>ASCPGACVCYNEPKVTTSCPQQGLQAVPTGIPASSQRIFLHGNRISHVPAASFQSCRNLTILWLHSNALARIDAAAFTGLTLLEQLDLSDNAQLHVVDPTTFHGLGHLHTLHLDRCGLRELGPGLFRGLAALQYLYLQDNNLQALPDNTFRDLGNLTHLFLHGNRIPSVPEHAFRGLHSLDRLLLHQNHVARVHPHAFRDLGRLMTLYLFANNLSMLPAEVLMPLRSLQYLRLNDNPWVCDCRARPLWAWLQKFRGSSSEV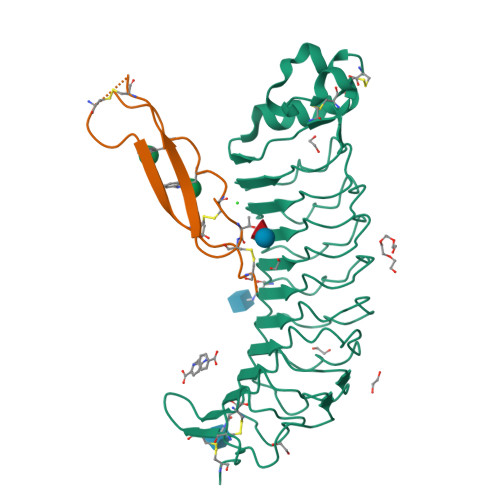PCNLPQRLADRDLKRLAASDLEGC[2x];>[2x]HGAWDEWSPWSLCSSTCGRGFRDRTRTCRPPQFGGNPCEGPEKQTKFCNIALCP>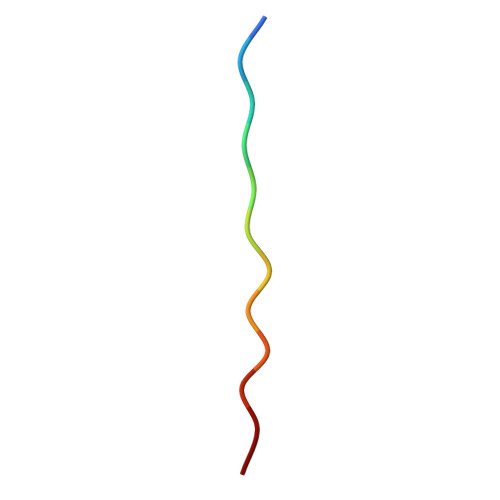 SEAAASTAVVIA>MRQVDAATHGGRAVIELREKILSGELPGGMRLFEVSTAELLDISRTPVREALSRLTEEGLLNRLPGGGFVVRRFGFADVVDAIEVRGVMEGTAARLAAERGVSKVALEEIDATVQQLDLCFGDRVDDVDFDGYAALNRIFHHQLAALCGSEMIRREVERASSLPFASPSAFLPDKANIGAFRRSLR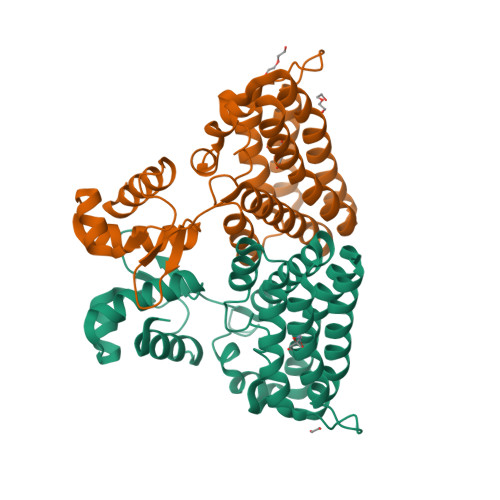GAQEQHKAIVAAIVAREGARAEAVAREHSRTARTNLEYMIREAPELIAQVPGLALISDHHHHHH[2x]>GINPFTMTTARDIMNAGVTCVGEHETLTAAAQYMREHDIGALPICGDDDRLHGMLTDRDIVIKGLAAGLDPNTATA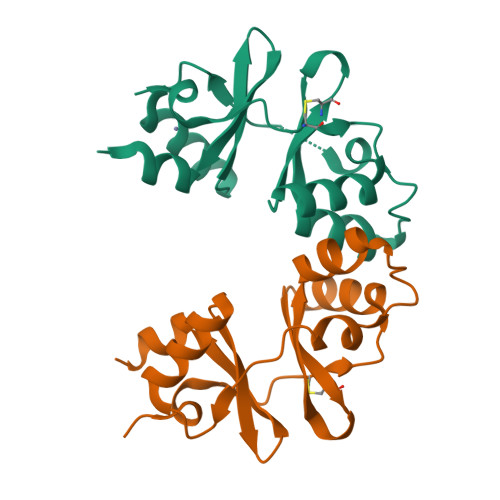GELARDSIYYVDANASIQEMLNVMEEHQVRRVPVISEHRLVGIVTEADIARHLPEHA[2x]D-glucuronic acid 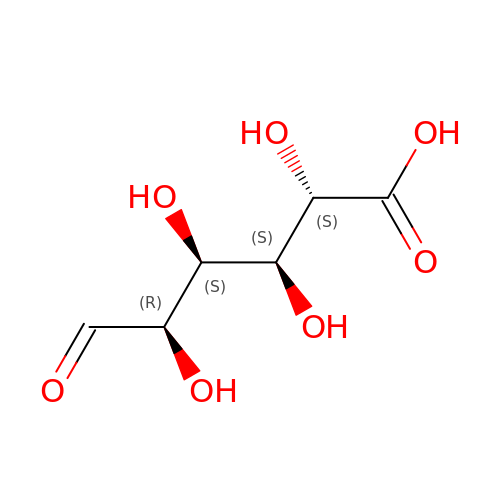| C6 H10 O7 | IAJILQKETJEXLJ-QTBDOELSSA-N>GSHMTELTYTEEVVSIEKLKEDDEFKTMVPSNNSREDLEKSLREKSQIFPLIADRNYVLIDGYTRLDI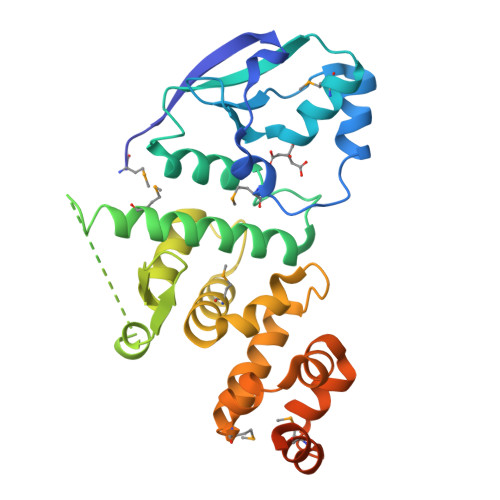MKKLGFKEVKILKYDFDSQQERDKAYELIWTFNGVRRQLDKNERLALFQKIADRIAKMQASKNKTEESKIVSHATQFSATESKQIEENEEFVTLDDGTTISALEYERILKELDKENKALSESDKRKMAILRINTPWLLKYVTDQKYKVPLDQAFRIYTRVKDMGILDKLKDLAPALRDPLITTREGRKIILNDEYRDLMEKIISKQYTTERAISVKQKEALKRGGKVKKSSK[3x]>GSHQEYIKKVADELKENSQNINDLLKEVEKNPEDMEYWNKIYRLLHTNKEIAETAGFSSVAKVEHTAMNLVDKMLNSEIKITSDLIDKIKKKVDMSTREIDKKV[2x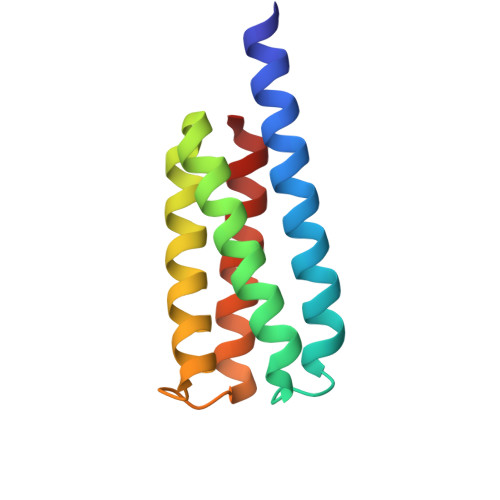]> MRIGHGFDVHAFGGEGPIIIGGVRIPYEKGLLAHSDGDVALHALTDALLGAAALGDI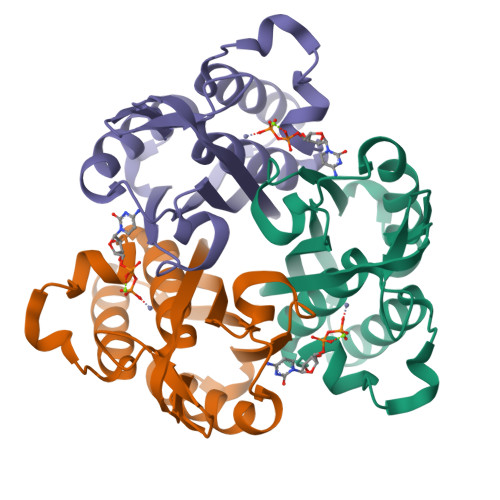GKLFPDTDPAFKGADSRELLREAWRRIQAKGYTLGNVDVTIIAQAPKMLPHIPQMRVFIAEDLGCHMDDVNVKATTTEKLGFTGRGEGIACEAVALLIKATK> GHTANKPCLAKFELLTSKWQMTSRKPPCV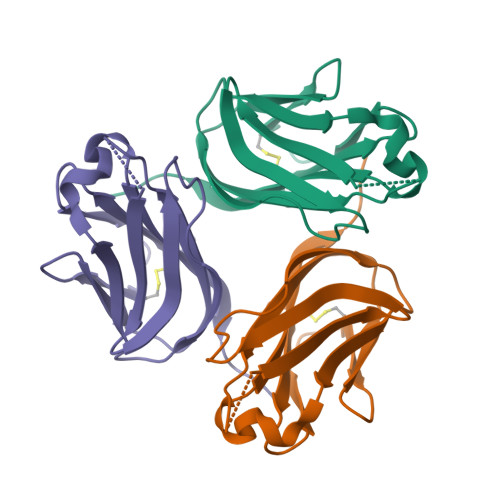NSLPEGKLKILQDGLYLIYGQVAPSTAYKGVAPFAVQLRKNEAMLQTLTSNSTIYDVGGTYEFHAGDIIDLIFDDEHQVLKNNTYWGIVLLANLFIS>MPREFKSFGSTEKSLLSKGHGEPSYSEIYAEPENFLEIEVHNPKTHIPNGMDSKGMFTDYEIICRTNLPSFHKRVSKVRRRYSDFEFFRKCLIKEISMLNHPKVMVPHLPGKILLSNRF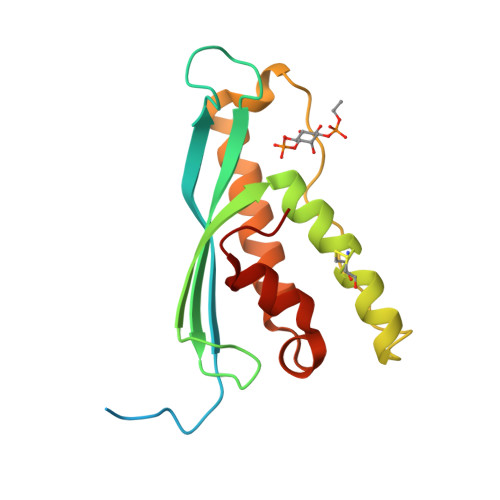SNEVIEERRQGLNTWMQSVAGHPLLQSGSKVLVRFIEAEKFVG[2x]>[2x]NPKSSLADGAHIGNYQIVKTLGEGSFGKVKLAYHTTTGQKVALKIINKKVLAKSDMQGRIEREISYLRLLRHPHIIKLYDVIKSKDEIIMVIEYAGNELFDYIVQRDKMSEQEARRFFQQIISAVEYCHRHKIVHRDLKPENLLLDEHLNVKIADFGLSNIMTDGNFLKTSCGSPNYAAPEVISGKLYAGPEVDVWSCG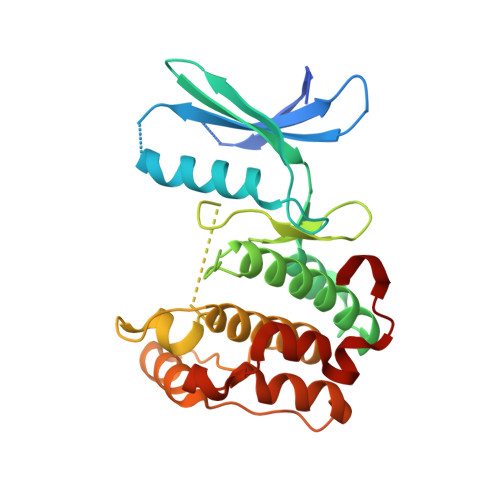VILYVMLCRRLPFDDESIPVLFKNISNGVYTLPKFLSPGAAGLIKRMLIVNPLNRISIHEIMQDDWFKVDLPEYLL Gemin5 in the Survival Motor Neuron (SMN) complex serves as the RNA-binding protein to deliver small nuclear RNAs (snRNAs) to the small nuclear ribonucleoprotein Sm complex via its N-terminal WD40 domain. Additionally, the C-terminal region plays an important role in regulating RNA translation by directly binding to viral RNAs and cellular mRNAs. Here, we present the three-dimensional structure of the Gemin5 C-terminal region, which adopts a homodecamer architecture comprised of a dimer of pentamers. By structural analysis, mutagenesis, and RNA-binding assays, we find that the intact pentamer/decamer is critical for the Gemin5 C-terminal region to bind cognate RNA ligands and to regulate mRNA translation.

To understand the mechanism underlying G5C self-assembly, we solved the structure of G5C by cryo-EM at an overall resolution of 3.31 Å based on the gold-standard Fourier shell correlation (FSC) curve. Consistent with the result from the SLS experiment, G5C forms a homodecamer with an MW of ~750 kDa. To our surprise, five G5C molecules (A–E or A’–E’) form a pentagon-like structure via its C-terminal region, named the pentamer region thereafter. Consistent with the previously solved TPR dimer structure, A–E forms homodimers with A’–E’. Thus, 10 G5C molecules assemble into a decamer comprised of a dimer of pentamers. The distance between the two parallel pentagon planes is ~177 Å with a rotation angle of 36°, and the rotation angle between the projections of two protomers in a TPR dimer, such as A and A’, is 108°. At the protomer–protomer interface of the G5C pentamer, an intermolecular five-helix bundle is formed by α28 and α29 of one protomer (molecule A, red) and α26, α31, and α32 of another protomer (molecule B, cyan), mainly via hydrophobic interactions, with a total buried accessible surface area of ~1400 Å2. In addition to hydrophobic interactions, intermolecular hydrogen bonds or salt bridges are found between Gln1378A side chain amide and Ser1472B main chain carbonyl and between Gln1389A side chain amide and Glu1462B side chain carboxyl. In the structure of the G5C decamer, two G5C dimers are spaced apart from each other, with the RBS1 of one G5C molecule (molecule C) spatially proximal to the positively charged surface of another molecule (molecule B), such that a large positively charged concave surface comprises residues from RBS1C and TPRB. Several basic residues of TPRB, including R1035, K1061, K1062, and R1090, are spatially close to RBS1C around the unstructured region between helices α26C and α27C.

>[10x]GHMKKRKARSLLPLSTSLDHRSKEELHQDCLVLATAKHSRELNEDVSADVEERFHLGLFTDRATLYRMIDIEGKGHLENGHPELFHQLMLWKGDLKGVLQTAAERGELTDNLVAMAPAAGYHVWLWAVEAFAKQLCFQDQYVKAASHLLSIHKVYEAVELLKSNHFYREAIAIAKARLRPEDPVLKDLYLSWGTVLERDGHYAVAAKCYLGATCAYDAAKVLAKKGDAASLRTAAELAAIVGEDELSASLALRCAQELLLANNWVGAQEALQLHESLQGQRLVFCLLELLSRHLEEKQLSEGKSSSSYHTWNTGTEGPFVERVTAVWKSIFSLDTPEQYQEAFQKLQNIKYPSATNNTPAKQLLLHICHDLTLAVLSQQMASWDEAVQALLRAVVRSYDSGSFTIMQEVYSAFLPDGCDHLRDKLGDHQSPATPAFKSLEAFFLYGRLYEFWWSLSRPCPNSSVWVRAGHRTLSVEPSQQLDTASTEETDPETSQPEPNRPSELDLRLTEEGERMLSTFKELFSEKHASLQNSQRTVAEVQETLAEMIRQHQKSQLCKSTANGPDKNEPEVEAEQPLCSSQSQCKEEKNEPLSLPELTKRLTEANQRMAKFPESIKAWPFPDVLECCLVLLLIRSHFPGCLAQEMQQQAQELLQKYGNTKTYRRHCQTFCM> GPLGSKNAPSTAGLGYGSWEIDPKDLTFLKELGTGQFGVVKYGKWRGQYDVAIKMIKEGSMSEDEFIEEAKVMMNLSHEKLVQLYGVCTKQRPIFII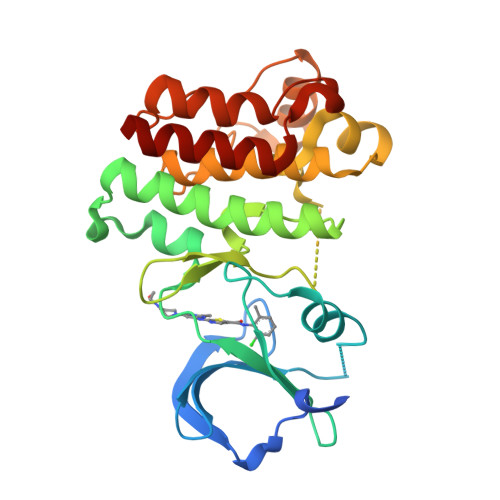TEYMANGCLLNYLREMRHRFQTQQLLEMCKDVCEAMEYLESKQFLHRDLAARNCLVNDQGVVKVSDFGLSRYVLDDEETSSVGSKFPVRWSPPEVLMYSKFSSKSDIWAFGVLMWEIYSLGKMPYERFTNSETAEHIAQGLRLYRPHLASEKVYTIMYSCWHEKADERPTFKILLSNILDVMDEES>[2x]MGSITENTSWNKEFSAEAVNGVFVLCKSSSKSCATNDLARASKEYLPASTFKIP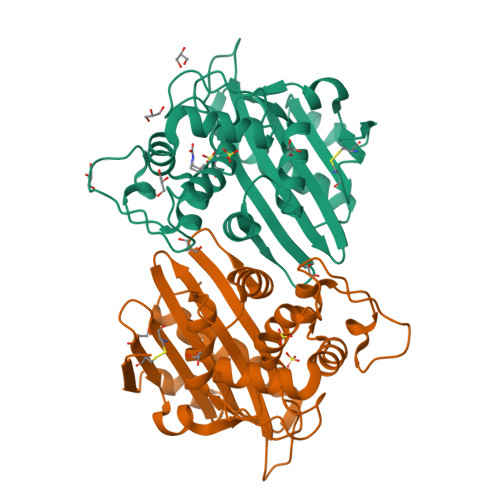NAIIGLETGVIKNEHQVFKWDGKPRAMKQWERDLTLRGAIQVSATPVFQQIAREVGEVRMQKYLKKFSYGNQNISGGIDKFWLEGQLRISAVNQVEFLESLYLNKLSASKENQLIVKEALVTEAAPEYLVHSKTGFSGVGTESNPGVAWWVGWVEKETEVYFFAFNMDIDNESKLPLRKSIPTKIMESEGIIGG L-glycero-alpha-D-manno-heptopyranose 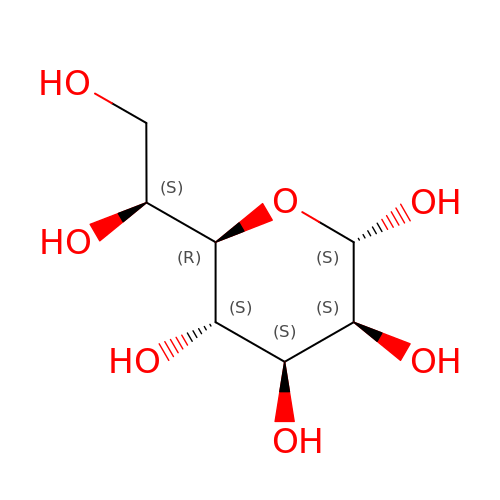| C7 H14 O7 | BGWQRWREUZVRGI-QQABCQGCSA-N> MEGEKGSKTRKGDALAREKLLEIAEKIYNQFEEEVVPSVSLPSRTKANLEYSDESDVWVYGDRESERSAKTVKGAFQLLKTTYATDFLINEHLARNRGSTLRELYYISEGWDYAKFKEQGESDRLIEDLEILTSLQREYFHMRPEEDGATMFGPIE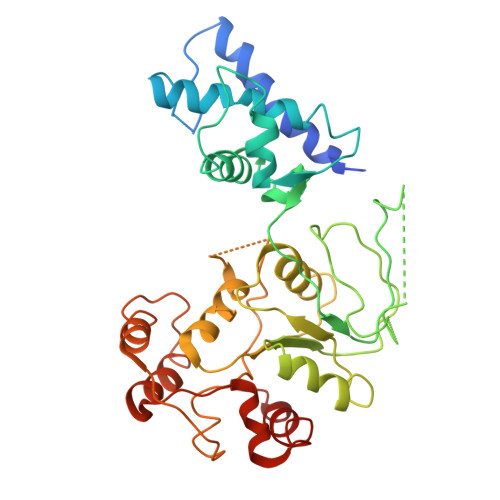ITEQTKRGERNIHCQKDVGEGGYQIPFNVENIEFQKHDASMIIAIETGGMYARLMENGFDEAYNAILVHLKGQPARSTRRIIKRMNEELGIPVAVFTDGDPWSYRIYASVAYGAIKSAHLSEFMATPAAKFLGLQPSDIVEYELSTDKLTEQDVSALRSELSDPRFESDYWKEQIQLQLDIGKKAEQQAFAGKGLDFVTEVYLPNRLKEMGMI> MAYNENDFKYFDDIRPFLDEIYKTRERYTPFYDDRADYNTNSKSYYDYISRLSKLIEVLARRIWDYDNELKKRFKNWDDLMKAFPEQAKDLFRGWLNDGTIDSIIHDEFKKYSAGLTSAFALFKVTEMKQMNDFKSEVKDLIKDIDRFVNGFELNELEPKFVMGFGGIRNAVNQSINIDKETNHMYSTQSDSQKPEGFWINKLTPSGDLISSMRIVQGGHGTTIGLERQSNGEMKIWLHHDGVAKLL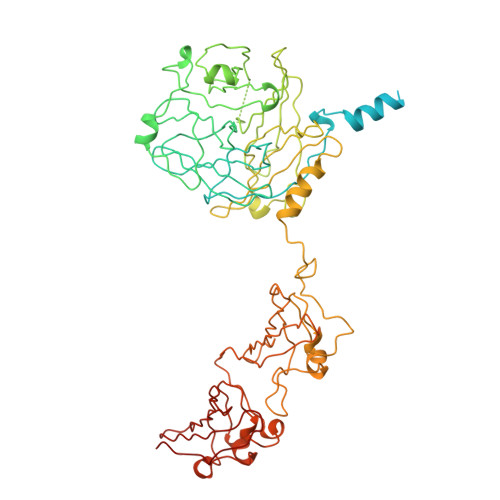QVAYKDNYVLDLEEAKGLTDYTPQSLLNKHTFTPLIDEANDKLILRFGDGTIQVRSRADVKNHIDNVEKEMTIDNSENNDNRWMQGIAVDGDDLYWLSGNSSVNSHVQIGKYSLTTGQKIYDYPFKLSYQDGINFPRDNFKEPEGICIYTNPKTKRKSLLLAMTNGGGGKRFHNLYGFFQLGEYEHFEALRARGSQNYKLTKDDGRALSIPDHIDDLNDLTQAGFYYIDGGTAEKLKNMPMNGSKRIIDAGCFINVYPTTQTLGTVQELTRFSTGRKMVKMVRGMTLDVFTLKWDYGLWTTIKTDAPYQEYLEASQYNNWIAYVTTAGEYYITGNQMELFRDAPEEIKKVGAWLRVSSGNAVGEVRQTLEANISEYKEFFSNVNAETKHREYGWVAKHQK> TTPLVHVASVEKGRSYEDFQKVYNAIALKLREDDEYDNYIGYGPVLVRLAWYTSGTWDKHDNTGGSYGGTYRFKKEFNDPSNAGLQNGFKFLEPIHKEFPWISSGDLFSLGGVTAVQEMQGPKIPWRCGRVDTPEDTTPDNGRLPDADKDADYVRTFFQRLNMNDREVVALMGAHALGKTHLKNSGYEGPWGAANNVFTNEFYLNLLNEDWKLEKNDA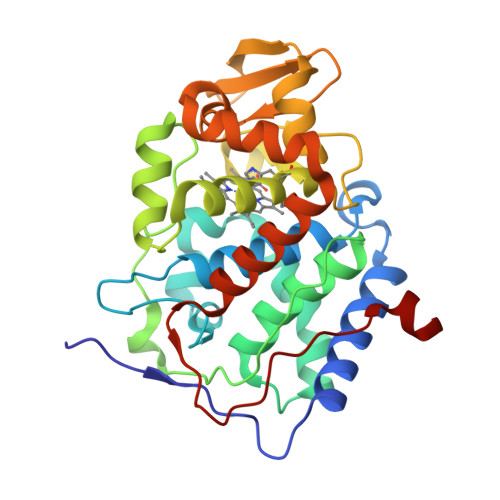NNEQWDSKSGYMMLPTDYSLIQDPKYLSIVKEYANDQDKFFKDFSKAFEKLLENGITFPKDAPSPFIFKTLEEQGL> MALVFVYGTLKRGQPNHRVLRDGAHG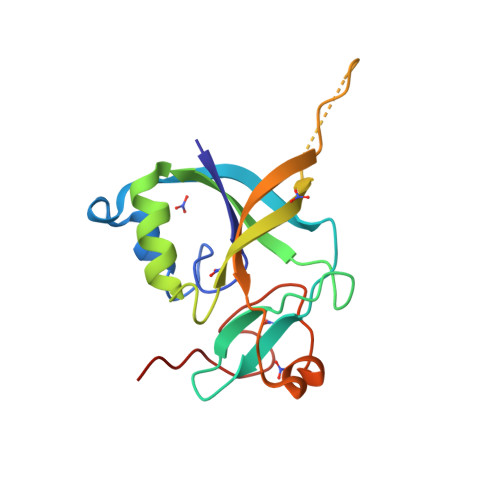SAAFRARGRTLEPYPLVIAGEHNIPWLLHLPGSGRLVEGEVYAVDERMLRFLDDFESCPALYQRTVLRVQLLEDRAPGAEEPPAPTAVQCFVYSRATFPPEWAQLPHHDSYDSEGPHGLRYNPRENR heptyl 4-deoxy-4-fluoro-alpha-D-mannopyranoside | 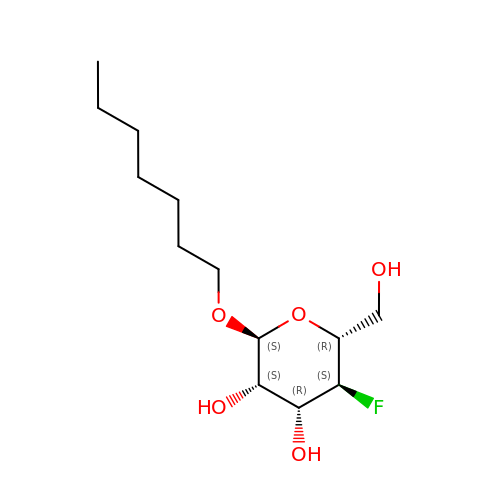C13 H25 F O5 | LFNSXYUDVVAWRK-BNDIWNMDSA-N~{N}1-[(~{S})-(3-chlorophenyl)-pyridin-2-yl-methyl]-4-methylsulfonyl-~{N}2-pyrimidin-2-yl-benzene-1,2-diamine 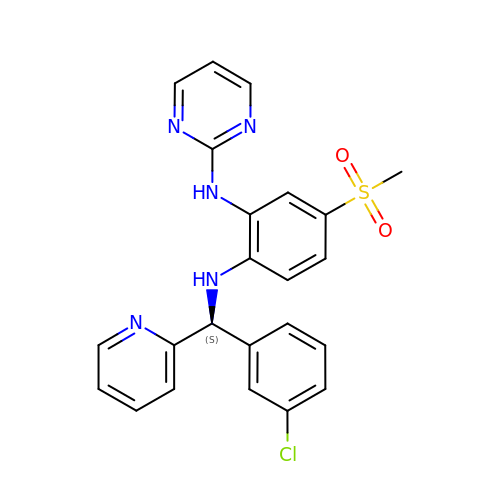| C23 H20 Cl N5 O2 S | JZZKDASEJHKEGM-QFIPXVFZSA-N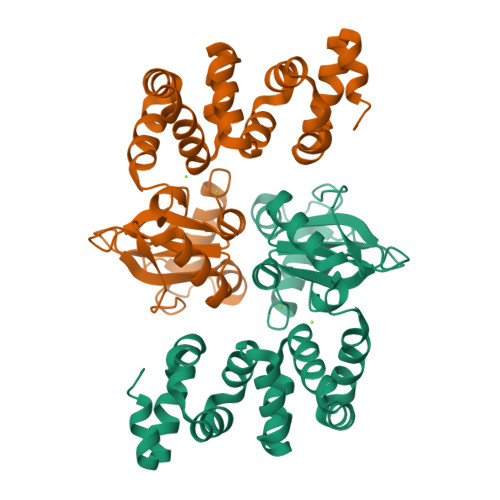> GSHMEEKLAVSLQEALQEGDTRALREVLEEIHPQDLLALWDELKGEHRYVVLTLLPKAKAAEVLSHLSPEEQAEYLKTLPPWRLREILEELSLDDLADALQAVRKEDPAYFQRLKDLLDPRTRAEVEALARYEEDEAGGLMTPEYVAVREGMTVEEVLRFLRRAAPDAETIYYIYVVDEKGRLKGVLSLRDLIVADPRTRVAEIMNPKVVYVRTDTDQEEVARLMADYDFTVLPVVDEEGRLVGIVTVDDVLDVLEAEATEDIHKLGAVDVPDLVYSE> GGACCGAUGAAGCUAGUGGAUGAGGUGUGACAAGCCGCCUAGCCAUACGACUCUUAAUAACUACUAUGACGAAAUAUACGGAUACGUUUAUUUUUUCUAAUUUCCACUUGGGUAGUACUAAUUGGGAGCAACGAAAAAAGUUGUGUAGAGAGAAGCAAGGGGACUCAUAUCUGAAACUAAGACACUUGCCGUCAGGGAUUCGCAAUAUGCCAUCUUCAGUUAAUUAAGGCUGAUUACCUUAGGAACCAAAAGAAGAAUAUCAACUAAGAAUUCGUGUCGUGAAGUUGUGGUGACGCAACUAUAACUGACGAGUAAGGUUUGAGUAGCCAAAAUCGACAAUCUUACAUUAACUGGAACAUUGCACAUGUUUGGUGAAAAUUGGAUAGGAAAAGAUCUAUGCCCUGAACUUGAAAUGCGGACU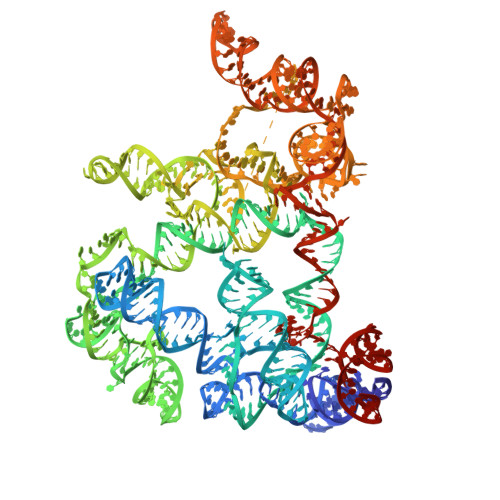AGGUCGUGGAAGUUGCUAGCCAUGAUGUGCUAGUCUGAUUCAGUAGUCUAAUAAGUCCAGAUACAAGAGUAUCCCACGUAAGCCAAUACGCGUCGGUUU Here, we describe the structure of trehalose-6-phosphate phosphatase (T6PP) from Brugia malayi. This enzyme is essential to the organism; deletion of the gene encoding T6PP results in toxic accumulation of trehalose 6-phosphate. The synthase catalyzes the condensation of glucose 6-phosphate and UDP-glucose, forming trehalose 6-phosphate, and T6PP catalyzes phosphoryl transfer to water, forming trehalose. The overall T6PP structure consists of a three-helix bundle N-terminal domain (residues 63–157) connected via a short linker (residues 158–205) to the Rossmann-fold catalytic core domain (residues 206–292; 398–492) and the α,β-fold cap domain (residues 293–397), which together comprise the HADSF phosphatase structure.

The structure of B. malayi T6PP bound to Mg2+ was determined at 3.0 Å resolution (residues 63–491). Electron density was not observed for residues 1–62 and SDS-PAGE analysis of dissolved crystals revealed that this region was not lost during crystallization. Thus, we conclude that residues 1–62 are probably disordered and are not required for stability or catalytic activity. A single magnesium ion is observed to be coordinated in the active site by two waters and four residues (Motif I: Asp213, Asp215 (mainchain C = O oxygen), Motif IV: Asp424 and Asp428). In B. malayi T6PP, the cap was found to be in an open orientation relative to the core, though the crystal contacts were consistent with stabilization of the protein in this conformation and the protein may exist in alternate conformations in solution. Notably, the B. malayi T6PP has a slightly more open conformation than the orthologous T. acidophilum enzyme. The MIT-like domain is tethered to the core domain by a helical-connector (residues 158–206) that is comprised of a broken α-helix (helices 4 and 5), which interacts with both domains and a second, longer α-helix (helix 6), which selectively interacts with the core domain. In T6PP, an intramolecular interaction occurs at the interface between the first and third α-helices of the MIT-like domain and the C1-loop of the HAD core domain, leaving the solvent-exposed interface between the second and third helices free to make intermolecular interactions with other proteins. Although the cap-open, unliganded form was observed in the structure, site-directed mutagenesis coupled with substrate and inhibition kinetics identified five residues important for catalysis and/or substrate affinity. Notably, no single residue is critical to binding, consistent with a mode of binding of the trehalose moiety by van der Waals contacts and shape complementarity between the sugar and enzyme.

> MGSSHHHHHHSSGGENLYFQGHMTETVTDQGKQRSSKLQKNEAAKDEQVEGKGKETLESGTDKSAEQNSSLLVGQPDVIDNDNVQTVDDFKNLMYKMQETRRAIVFALLNEKDLTKDDVEILKRAYEKLTDNQTHSFQREMCTLTTKLSVNIGDETRGLEKDLKYLDALMNIRREEPNLLWPIIMSRVDLFSILANYHPKGKETFLKEYEDTVKFLKTFISSEAITGKKPIFITDWDGTMKDYCSQYATNLQPVYSAVGMTRFAASFTRISAVLTAGPLRGPGILDLTAMPIDGPVMFSGSWGREWWLSGKRVVHQDGITDEGFNALQRLDDEMKDLLHTSDYAPFALVGSGVQRKVDRLTLGVQTVCHHVTSELSNRYQMAVKERMHRVDPNSQILVFDPSTELEVEVVAHNSGIIWNKGNGVERLIKSLGDSLQSPGKILICGDTLSDIPMVRQAVKQNPDGVLAIFVGAKMSLREEVKQVIGDESRCCFVSCPDVIHAAMSQILNEHCIGK> AGAQDFVPHTADLAELAAAAGECRGCGLYRDATQAVFGAGGRSARIMMIGEQPGDKEDLAGLPFVGPAGRLLDRALEAADIDRDALYVTNAVKHFKFTRAAGGKRRIGKTPSRTEVVACRPWLIAEMTSVEPDVVVLLGATAAKALLGNDFRVTQHRGEVLHVDDVPGDPALVATVHPSSLLRGPKEERESAFAGLVDDLRVAADVR

UdgX excises uracil from uracil-containing DNA to concurrently form a covalent bond with the resulting AP-DNA. Structurally, UdgX is highly similar to family-4 UDGs (F4-UDGs). However, UdgX is unique in possessing a flexible R-loop (105KRRIH109). Our earlier studies allowed us to propose a reaction mechanism of UdgX, which involves the formation of a covalent bond between H109 of UdgX with the C1′ position of the target deoxyribose sugar concurrently with the uracil excision from this site in DNA.

Substitutions of His109 in MsmUdgX with Ser, Gly, Ala, Gln, Cys and Lys showed the loss of its covalent complex formation with DNA but gained canonical UDG activities. In the reactions of the mutant proteins with ssU9, the entire substrate was converted to product by the H109G mutant, while hardly any substrate was utilized by the H109K mutant. We note that smaller and hydrophilic amino acid substitutions at His109, such as Gly or Ser showed higher Kcat/Km values. Further, the overlay of all the structures of UdgX H109 mutants showed that the overall structures are very well conserved with a Cα RMSD of ca 0.2 Å. As anticipated, we note a clear difference in the sizes of the active site cavities in the various mutants. When we arranged the mutants in the order of increasing cavity sizes (left), we noted that the canonical UDG activity of the mutants increased with their increasing cavity sizes to begin with and then with a further increase in the cavity size, the UDG activity declined (right). It suggested that the initial increase in UDG activity (H109K to H109Q to H109G) occurred because of the efficiency with which the water molecule could be localized to make a nucleophilic attack on the C1′ position. Interestingly, G109 the smallest amino acid substitution of H109 showed lower cavity volume than Ser, Cys or Ala due to an overall structural change near the active site.> GHMSYNGIRIGQGYDIHKIKVLDEEYNTYANNDFNKNEQSFKTLTLGGVKINNVLVLSHSDGDIIYHSIVDSILGALGSLDIGTLFPDKDEKNKNKNSAIFLRYARLLIYKKNYDIGNVDINVIAQVPKISNIRKNIIKNISTVLNIDESQISVKGKTHEKLGVIGEKKAIECFANILLIPKNS

2C-methyl-D-erythritol-2,4-cyclodiphosphate synthase (IspF) catalyzes the conversion of 4-diphosphocytidyl-2C-methyl-D-erythritol-2-phosphate to 2C-methyl-D-erythritol-2,4-cyclodiphosphate and cytidine monophosphate in production of isoprenoid-precursors via the methylerythritol phosphate biosynthetic pathway. IspF represents a potential target for development of broad-spectrum antimicrobial drugs since it is proven or inferred as essential in these pathogens and absent from mammals. In all IspF crystal structures three subunits form a compact bell-shaped assembly approximately 45 Å by 60 Å in the axial and equatorial dimensions respectively. The enzyme active site is located in a cleft at the interface of two subunits and here Zn2+ is coordinated by the side chains of two histidines and an aspartate.

One subunit is present in the asymmetric unit of PfIspF and the trimer is generated by the symmetry operations (−x + y, -x, z) and (−y, x-y, z). PfIspF contains a 19 residue insertion at the N-terminus, Lys76 - Glu94, immediately after β1 that does not align with bacterial IspF sequences. Here, residues Tyr82 - Phe97 could not be modeled due to the lack of ordered electron density. The coordinating residues are Asp10, His12 and His44 in BcIspF, Asp71, His73 and His123 in PfIspF. The structure-based sequence alignment and overlay of the active sites of BcIspF:CMP and PfIspF:CDP complexes indicate that the key enzyme-ligand interactions and aspects of the structure that are implicated in substrate specificity and the mechanism are highly conserved. Note that in the PfIspF:CDP complex two conformers of CDP are present that differ in the orientation of the β-phosphate group. These refined satisfactorily at occupancy levels of 0.6 and 0.4. Similarly in PfIspF side chains of Tyr70, Ile72, Ile180 and Val220 line this cavity, and the side chains of Phe230 form the floor of the cavity. In PfIspF, a sulfate binds close to this site but dislodged such that anion coordination involves the main chain amides of nearby residues, Val220 from all three subunits, rather than a basic side chain. Since there are no pronounced differences between the CDP bound and unliganded PfIspF structures only the former is discussed.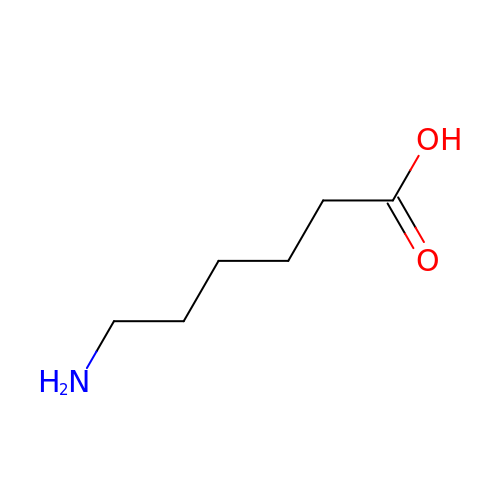6-AMINOHEXANOIC ACID | C6 H13 N O2 | SLXKOJJOQWFEFD-UHFFFAOYSA-N>GGDPHMMFGKKKNNGGSSTARYSAGNKYNTLSNNYALSAQQLLNASKIDDIDSMMGFERYVPPQYNGRFDAKDIDQIPGRVGWLTNMHATLVSQETLSSGSNGGGNSNDGERVTTNQGISGVDFYFLDEEGGSFKSTVVYDPYFFIACNDESRVNDVEELVKKYLESCLKSLQIIRKEDLTMDNHLLGLQKTLIKLSFVNSNQLFEARKLLRPILQDNANNNVQRNIYNVAANGSEKVDAKHLIEDIREYDVPYHVRVSIDKDIRVGKWYKVTQQGFIEDTRKIAFADPVVMAFAIATTKPPLKFPDSAVDQIMMISYMIDGEGFLITNREIISEDIEDFEYTPKPEYPGFFTIFNENDEVALLQRFFEHIRDVRPTVISTFNGDFFDWPFIHNRSKIHGLDMFDEIGFAPDAEGEYKSSYCSHMDCFRWVKRDSYLPQGSQGLKAVTQSKLGYNPIELDPELMTPYAFEKPQHLSEYSVSDAVATYYLYMKYVHPFIFSLCTIIPLNPDETLRKGTGTLCEMLLMVQAYQHNILLPNKHTDPIERFYDGHLLESETYVGGHVESLEAGVFRSDLKNEFKIDPSAIDELLQELPEALKFSVEVENKSSVDKVTNFEEIKNQITQKLLELKENNIRNELPLIYHVDVASGYPNIMTTNRLQPDSIKAERDCASCDFNRPGKTCARKLKWAWRGEFFPSKMDEYNMIKRALQNETFPNKNKFSKKKVLTFDELSYADQVIHIKKRLTEYSRKVYHRVKVSEIVEREAIVCQRENPFYVDTVKSFRDRRYEFKGLAKTWKGNLSKIDPSDKHARDEAKKMIVLYDSLQLAHKVILNSFYGYVMRKGSRWYSMEMAGITCLTGATIIQMARALVERVGRPLELDTDGIWCILPKSFPETYFFTLENGKKLYLSYPCSMLNYRVHQKFTNHQYQELKDPLNYIYETHSENTIFFEVDGPYKAMILPSSKEEGKGIKKRYAVFNEDGSLAELKGFELKRRGELQLIKNFQSDIFKVFLEGDTLEGCYSAVASVCNRWLDVLDSHGLMLEDEDLVSLICENRSMSKTLKEYEGQKSTSITTARRLGDFLGEDMVKDKGLQCKYIISSKPFNAPVTERAIPVAIFSADIPIKRSFLRRWTLDPSLEDLDIRTIIDWGYYRERLGSAIQKIITIPAALQGVSNPVPRVEHPDWLKRKIAT[2x]

The Saccharomyces cerevisiae B-family replicative DNA polymerases, namely Pol ϵ, Pol δ and Pol α, have been estimated to incorporate about 13 000 NTPs during each cell cycle of the yeast genome, and Pol ϵ seems to incorporate the majority of NTPs, roughly four times as many ribonucleotides as Pol δ. Other examples where an amino acid adjacent to the steric gate residue influences ribonucleotide discrimination are found among B-family polymerases. It was first shown in the ϕ29 DNA polymerase that B-family polymerases have a conserved tyrosine (Y645 in Pol ϵ) that functions as a steric gate. Our data show that Pol ϵ discriminates NTPs through the concerted action of a steric gate residue (Y645) and a sensor in the finger domain (N828). A comparison with other B-family DNA polymerases showed that both Y645 and N828 are structurally conserved residues, thus reinforcing their functional importance.

A series of crystal structures were determined of M644GPol2CORE (the catalytic domain of Pol ϵ (136 kDa)) in complex with dTTP or UTP and dCTP or CTP opposite the template dA and dG, respectively. The described structural changes were also found when comparing M644GPol2CORE-CTP with M644GPol2CORE-dCTP. However, a small ∼1Å shift in the backbone Cα-atom of the catalytic residue D877 towards the cavity between D877 and Y645 was consistently observed in all M644GPol2CORE structures when compared to wild-type Pol2CORE structures. This consistent structural shift in D877 suggests increased flexibility at the polymerase active site of M644GPol2CORE, something that was hypothesized when M644GPol2CORE was created for use in earlier studies. A deoxyribonucleotide has a perfect fit and stacks on the steric gate residue while N828 in the finger domain forms a loose hydrogen bond with the β-phosphate of the deoxyribonucleotide.The non-LEE encoded effector protein B (NleB) has GT activity and inhibits NF-κB activation by transferring N-acetyl glucosamine (GlcNAc) to host death domain-containing proteins and to glyceraldehyde 3-phosphate dehydrogenase (GAPDH). The glycosylation target is an arginine residue, which was unexpected because the guanidine group of arginine is nucleophilically poor at physiological pH. The T3SS effectors SseK1 and SseK2 from Salmonella typhimurium SL1344 are NleB orthologs that behave as NleB1-like GTs, although they differ in protein substrate specificity. Here, by using a combination of X-ray crystallography, STD-NMR, enzyme kinetics, molecular dynamics simulations, and in vivo experiments, we show that these enzymes are GT-A fold retaining GTs that most likely follow an SNi mechanism.

We solved the crystal structures of Salmonella enterica serovar Typhimurium SL1344 SseK1 in complex with UDP. Point mutations (C39S, C210S) were introduced into SseK1 to prevent protein precipitation due to irregular intermolecular disulfide binding. However, in the sandwich-like π-π stacking, the interaction modes of SseK1 and SseK2 are slightly different. In contrast to SseK2, Trp331 from the C-terminal lid of SseK1 interacts with the uracil base instead of Phe203 (second and third panels). While the Kd measured for binding of UDP-GlcNAc to SseK1 F187A was similar to wild type SseK1, the Kd for binding of UDP-GlcNAc to SseK2 F203A was increased about 13-fold as compared to wild type SseK2. These data suggest that although the sandwich-like π-π stacking interactions are maintained, the uracil binding modes within SseK1 and SseK2 are slightly different. The conserved arginine residue in SseK2 and SseK3 (Arg348SseK2, Arg335SseK3), which is located in the lid domain, is substituted to an alanine residue in SseK1 (Ala332SseK1). In the crystal structure of UDP-bound SseK1, the backbone direction of Ala332 is located at the opposite side of UDP. This implies that the lid domain of SseK1 is likely more flexible than SseK2 and SseK3. The arginine on the C-terminus participates in an interaction with UDP-GlcNAc in SseK2 and SseK3, but not in SseK1. Based on this result, the departure of the leaving group is likely to be easier, due to a weaker enzyme-substrate interaction network in SseK1, than in SseK2 and SesK3.

> MIPPLNRYVPALSKNELVKTVTNRDIQFTSFNGKDYPLCFLDEKTPLLFQWFERNPARFGKNDIPIINTEKNPYLNNIIKAATIEKERLIGIFVDGDFFPGQKDAFSKLEYDYENIKVIYRNDIDFSMYDKKLSEIYMENISKQESMPEEKRDCHLLQLLKKELSDIQEGNDSLIKSYLLDKGHGWFDFYRNMAMLKAGQLFLEADKVGCYDLSTNSGCIYLDADMIITEKLGGIYIPDGIAVHVERIDGRASMENGIIAVDRNNHPALLAGLEIMHTKFDADPYSDGVCNGIRKHFNYSLNEDYNSFCDFIEFKHDNIIMNTSQFTQSSWARHVQ> MPQIPTMKILIDENMPYAQALFSQLGEVILKPGRTLTADDLIDVDALMIRSVTKVNDALLAKANRLKFVGTATAGMDHVDQALLRERGIFFTAAPGCNKVGVAEYVFSVLMVLAQQQGFSVFDKTVGIIGAGQVGSYLAKCLSGIGMKVLLNDPPKQAQGDEREFTELETLLKQADVITLHTPITRGGE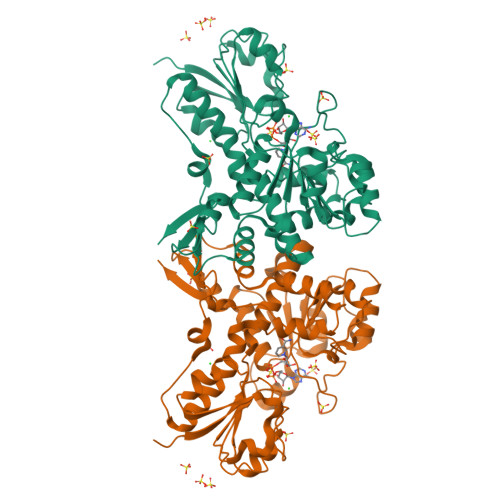WPTHHLIDAAILEQLRSDQILINAARGPVVDNAALKARLQQGDGFTAVLDVFEFEPQVDMELLPLLAFATPHIAGYGLEGKARGTTMIFNSYCEFLGSAHCANPASLLPKAPVPKVYLERAWDEETLRTLTQIIYDVRKDDAQFRREIHQPGAFDLMRKHYWDRREYSAVTLAGGADCHLAPLAKLGFQVEVCDEPTI>[2x]MFTGSIVAIVTPMDEKGNVCRASLKKLIDYHVASGTSAIVSVGVTGESATLNHDEHADVVMMTLDLADGRIPVIAGTGANATAEAISLTQRFNDSGIVGCLTVTPYYNRPSQEGLYQHFKAIAEHTDLPQILYNVPSRTGCDLLPETVGRLAKVKNIIGIKEATGNLTRVNQIKELVSDDFVLLSGDDASAL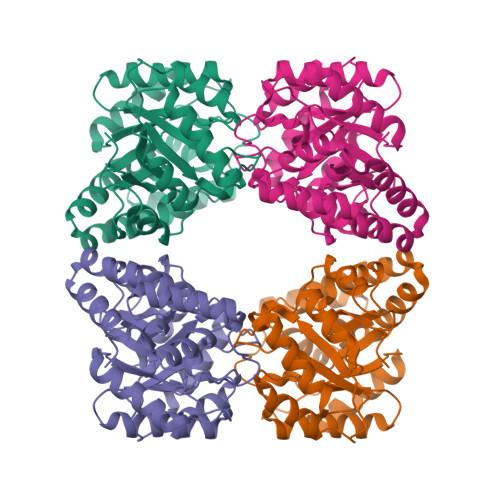DFMQLGGHGVISVTANVAARDMAQMCKLAAEGHFAEARVINQRLMPLHNKLFVEPNPIPVKWACKELGLVATDTLRLPMTPITDSGRETVRAALKHAGLL> SMS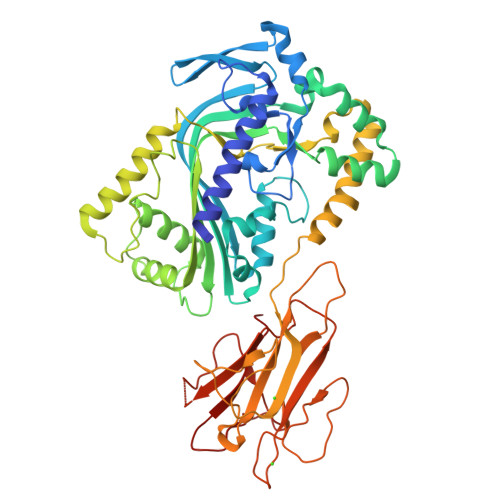NDKTGKSLEQENSERDVEIRDRNYFRKLSLFDDTVIAGAEMIGTSYDVFGKYCNVGSCMNSLFDERKINASEDNFKKVTILGKTLKVPYYIDCYSVGDLKYTNASGESIESYQSNISSKSRIKGNYLFFSASLKVDFDTDSLTDFENAFSRIQYTYDLYILKSSAEALKEFLKESVKTALDKADTEEDMNDLFNTWGSHFLSGVVMGGCAQYSSSTNKYTSNLTNSFDVVAAASFAGFIGLSARTGNSFMEDIKKFRSASNIKTHAIGGDLSRFDPFGGATSADQPSAEEIAAAKKAFEDWKASVPNAPELVNFADSNPLTGIWELCSDRTQKAKLKKHFETVWAPAESAKRRVHADYIDEIIIGINNTNTPPEGYIGLKSTKDENLNSKGNICLFMHKAKYDPNIDNKDCITELKFITVRDKSPEGDWVKIPQDIYISPNQYLYLCYLPAKYSAEKAIKDIQLLCSSCGSSMILPYGYNDVLDERGERANATEDDNVHYLIYSAGWK2-[2-[4-(4-methoxyphenyl)phenyl]sulfonylphenyl]-~{N}-oxidanyl-ethanamide | C21 H19 N O5 S | 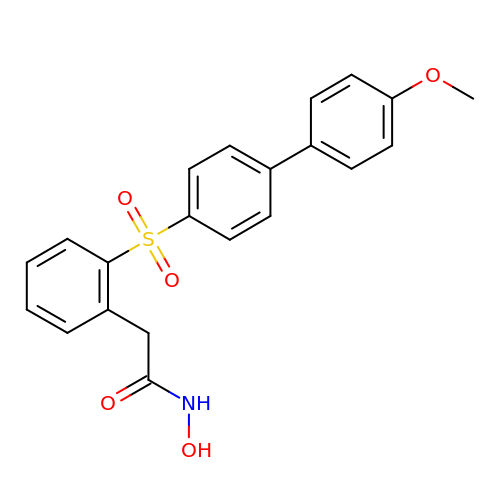DJZNIZCARKSSDE-UHFFFAOYSA-N>MGSSHHHHHHSSRNLYFQGGGHMFFLNLKQINDRFNTEFITKFKEILESGWYILGKQCEKFENNFAKYCGVKHCIGVANGLDALRLIIKAYDFKENDEIIVPANTYIASILAITDNKCKPILIEPDINTYNINPDLIEEKITKKTKAIMVVHLYGQVCDMEKIQLLANKYNLKIIEDCAQAHGAIYKDKRVGNLGDAAGFSFYPGKNLGALGDAGCICTNDDNFASKIRALANYGSHKKYENLYTGLNSRLDEIQAAFLDIKLKYLDEDNNKRKNIANFYLQN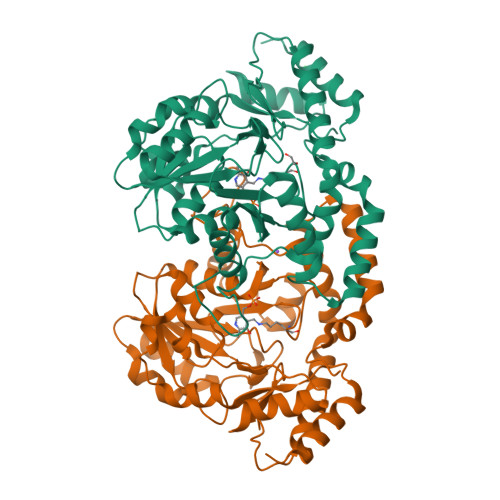IKNENIILPSNKFDHVWHLFVVKTKLRDELQHYLNNHDIQTIIHYPIPPHKQKCYKDLNHLKLPITENIHQEVLSLPISPTMKENDFKKVADILNKWKV[4x]>MEIRYTPKELTKLPRTVEYKNKSVYMINQRLLPKEFKVEKFSKVEEVAEAIKNMTVRGAPAIGAAAGFGLALYAETSKAKTKEEFL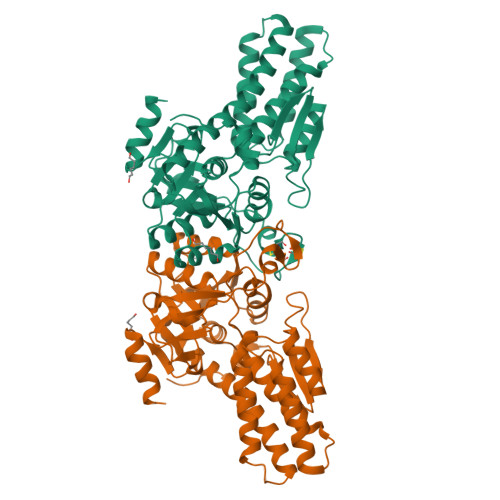DGFEKAYEILKNTRPTAVNLFWALNRIKKLVEEHSEDPLDEIKRLIVQEAYKIADEDVEANLRMGHYGAEVLPEGNILTHCNAGSLATVHLGTVGSVVRVMHKDGSLKLLWLDETRPVLQGARLSAWEYSYDGLNVKLIADNAAAFVMQQGFVDAIIVGADRIVANGDFANKIGTYMLAVLAREHGIPFFAVAPLSSIDMELKSGKDIPIEERSPEEVLTCGGCRIAPDVPVYNPAFDVTPHKYLTGIITDRGVVWPPFKRNLKKLFEVNKSGGDEAV[2x]>[2x]MNLVLMGLPGAGKGTQGERIVEDYGIPHISTGDMFRAAMKEETPLGLEAKSYIDKG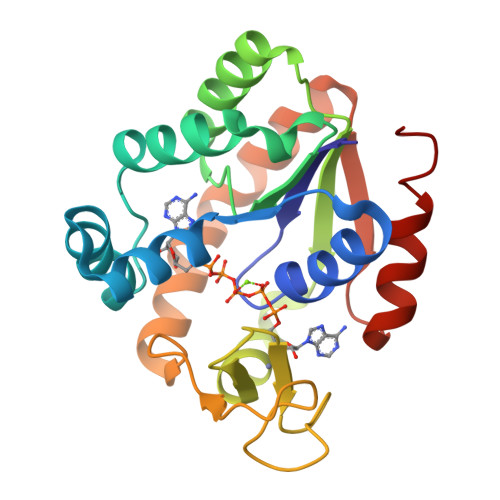ELVPDEVTIGIVKERLGKDDCERGFLLDGFPRTVAQAEALEEILEEYGKPIDYVINIEVDKDVLMERLTGRRICSVCGTTYHLVFNPPKTPGICDKDGGELYQRADDNEETVSKRLEVNMKQTQPLLDFYSEKGYLANVNGQRDIQDVYADVKDLLGGLK UNDECYLAMINE-N,N-DIMETHYL-N-OXIDE 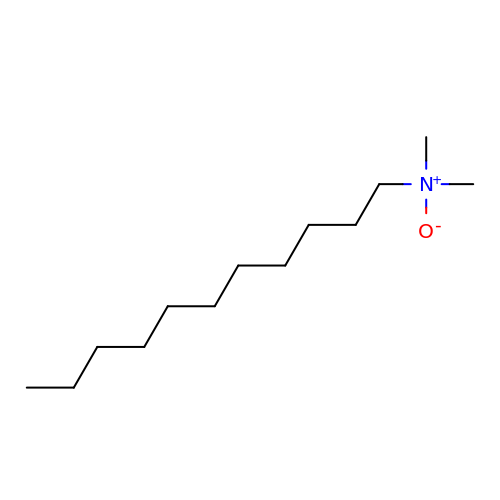| C13 H29 N O | OZHBUVQCJMARBN-UHFFFAOYSA-N> ADWDFSAISRKATALYGPLGAGQQRIDAWQNLLATQKQVSEMEKLKVVNLFFNKQMRYVEDIDLWHEVDYWETPIEALWKGAGDCEDYAIAKYFSLRHLGVASDKLRITYVKALRQNRAHMVLTYYSSPDAMPLVLDSLIDPI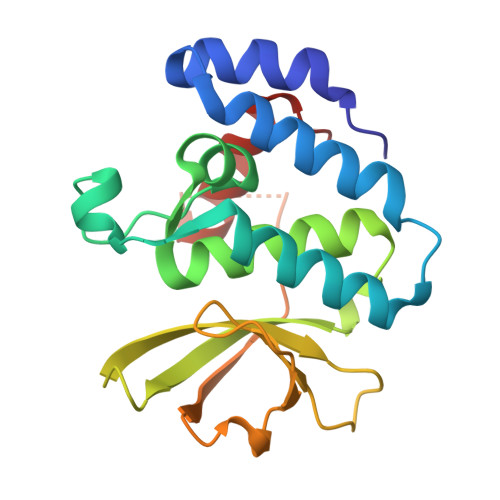KPAAERTDLLPVYSFNAEGLYLPGAKGNKKVGDTKRLSRWQDVLKKMQAEGFPV> GSHMKNSVSVDLPGSMKVLVSKSSNADGKYDLIATVDALELSGTSDKNNGSGVLEGVKADASKV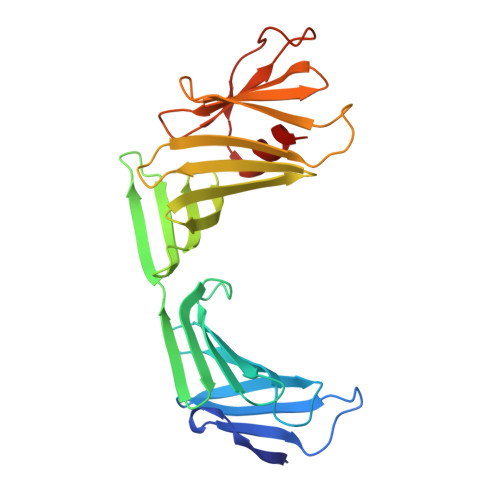KLTISDDLGQTTLEVFKSDGSTLVSKKVTSGGSSTEEKGGEKIITRADGTRLEYTGIKSDGSGKAKEVLKGYVLEGTLTAEKTTLVVKEGTVTLSKNISKSGEVSVELNDTDSSAATKKTAAWNSGTSTLTITVNSKKTKDLVFTSSNTITVQQYDSNGTSLEGSAVEITKLDEIKNALK>SNAMLINKTKRAEQNLNNLPFLALQAEQIEFLGSSAEFKTQIIELIRNAKKRIYVTALYWQKDEAGQEILDEIYRVKQENPHLDVKVLIDWHRAQRNLLGAEKSATNADWYCEQRQTYQLPDDPNMFFGVPINTREVFGVLHVKGFVFDDTVLYSGASINNVYLHQFEKYRYDRYQKITHAELADSMVNFINDYLLDFSAVYPLDVTNRPRTKEIRGNIRAYRKDLAQNGEYSLKSAVKLPNVLSVSPLFGLGASGNELNQVIEDLFLQVQKKLVICTPYFNFPRTLQHKIATLLENGKRVEIIVGDKVANDFYIPPEQPFKMAGALPYLYESNLRRFCEKFETQIESGQLVVRLWRDGDNTYHLKGVWVDDRYILLTGNNLNPRA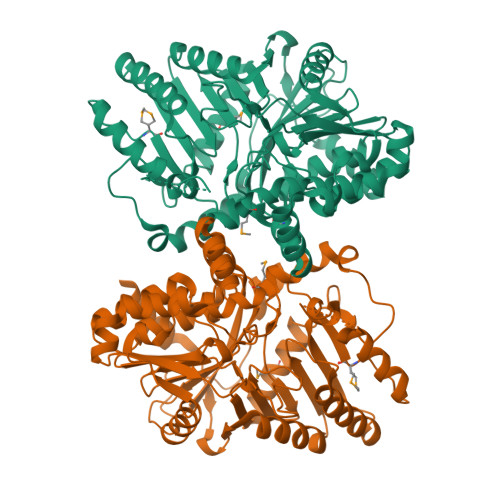WRLDAENGLLIYDPQQQLLAQVEKEQNQIRQHTKVLKHYTELEELNQYPEPVQKLLKKFARIKADKLVKMIL[3x]>[2x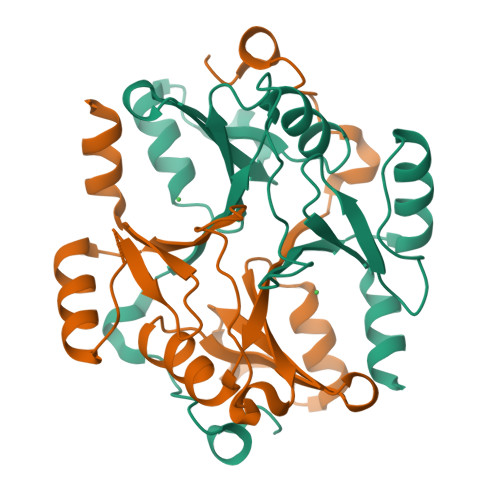]GAGAGAGAGAGMGSMDSKESPANNPGLHTPPDEATKGYIMQQTMFRIKDPKRTLEFYSRVLGMSLLNKVDVPYMKMTLYMMGYEDVSSAPSDPVEKTIWTFGRPATMELTHFWGTENDPEFKGYHNGNSEPIGFGHIGITVDDMYKACERFESLGVEFVKKPSDGYTFIKDPDGYWIEIFDLNGIRAIVNTL> MKLSSACAIALLAAQAAGASIKHRINGFTLTEHSDPAKRELLQKYVTWDDKSLFINGERIMIFSGEFHPFRLPVKELQLDIFQKVKALGFNCVSFYVDWALVEGKPGEYRADGIFDLEPFFDAASEAGIYLLARPGPYINAESSGGGFPGWLQRVNGTLRSSDKAYLDATDNYVSHVAATIAKYQITNGGPIILYQPENEYTSGCCGVEFPDPVYMQYVEDQARNAGVVIPLINNDASASGNNAPGTGKGAVDIYGHDSYPLGFDCANPTVWPSGDLPTNFRTLHLEQSPTTPYAIVEFQGGSYDPWGGPGFAACSELLNNEFERVFYKNDFSFQIAIMNLYMIFGGTNWGNLGYPNGYTSYDYGSAVTESRNITREKYSELKLLGNFAKVSPGYLTASPGNLTTSGYADTTDLTVTPLLGNSTGSFFVVRHSDYSSEESTSYKLRLPTSAGSVTIPQLGGTLTLNGRDSKIHVTDYNVSGTNIIYSTAEVFTWKKFADGKVLVLYGGAGEHHELAISTKSNVTVIEGSESGISSKQTSSSVVVGWDVSTTRRIIQVGDLKILLLDRNSAYNYWVPQLATDGTSPGFSTPEKVASSIIVKAGYLVRTAYLKGSGLYLTADFNATTSVEVIGVPSTAKNLFINGDKTSHTVDKNGIWSATVDYNAPDISLPSLKDLDWKYVDTLPEIQSSYDDSLWPAADLKQTKNTLRSLTTPTSLYSSDYGFHTGYLLYRGHFTATGNESTFAIDTQGGSAFGSSVWLNGTYLGSWTGLYANSDYNATYNLPQLQAGKTYVITVVIDNMGLEENWTVGEDLMKTPRGILNFLLAGRPSSAISWKLTGNLGGEDYEDK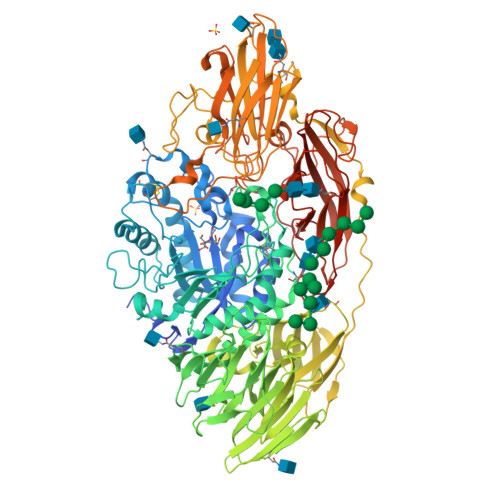VRGPLNEGGLYAERQGFHQPEPPSQNWKSSSPLEGLSEAGIGFYSASFDLDLPKGWDVPLFLNIGNSTTPSPYRVQVYVNGYQYAKYISNIGPQTSFPVPEGILNYRGTNWLAVTLWALDSAGGKLESLELSYTTPVLTALGEVESVDQPKYKKRKGAYHHHHHH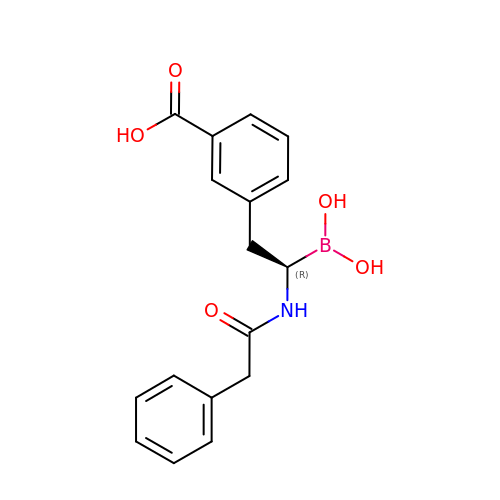(1R)-2-PHENYLACETAMIDO-2-(3-CARBOXYPHENYL)ETHYL BORONIC ACID | C17 H18 B N O5 | ZAHVYMBTUDWUAX-HNNXBMFYSA-N>MNDLIYQDEHASLQPLEGRTVAVIGYGIQGRAFAANLRDSGVAVRVGNIDDRYFELARAEGHRVTNIAEAVAHADIVLLLIPDEAHGAVFDVDIAPNLRDGALLCVAHGHSLVQGDVRPLPGRDLAMLAPRMYGDPIRRYYLAGQGAPAYFDIVADHTGRARDRVLAIARAVGFTRAGVMALGYRQETFLDLFQEQFLAPALVDLVETGFQVLVERGFNPKAALLEVYGSGEMGKMMLDGADIGLDEVVALQGSPTCQVGYHRWRGRTLPTAVREL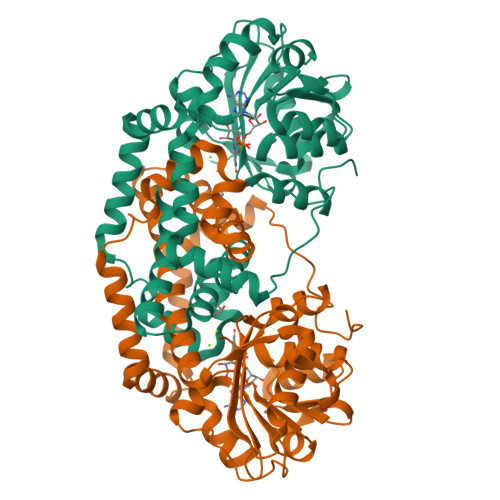AARVLDQIEGGDFSAYLKEQASNDYASLDDARRAALKRPLNVAHAQVRAAFRFPTEAAGGLYQAAQAPADVEPEAAR[2x]> GSHGWTSKGQITVLDMHPGSGKTHRVLPELIRQCIDRRLRTLVLAPTRVVLKE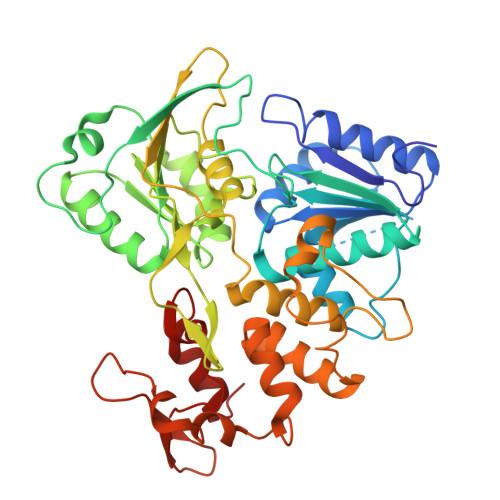MERALNGKRVRFHSPAVSDQQAGGAIVDVMCHATYVNRRLLPQGRQNWEVAIMDEAHWTDPHSIAARGHLYTLAKENKCALVLMTATPPGKSEPFPESNGAITSEERQIPNGEWRDGFDWITEYEGRTAWFVPSIAKGGAIARTLRQKGKSVICLNSKTFEKDYSRVRDEKPDFVVTTDISEMGANLDVSRVIDGRTNIKPEEVDGKVELTGTRRVTTASAAQRRGRVGRQDGRTDEYIYSGQCDDDDSGLVQWKEAQILLDNITTLRGPVATFYGPEQDKMPEVAGHFRLTEEKRKHFRHLLTHCDFTPWLAWHVAANVSSVTDRSWTWEGPEANAVDEASGGLVTFRSPNGAERTLRPVWKDARMFKEGRDIKEFVAYASGRR>[16x]ETGDKPLGETGTTGFQICKNALKLPVLEVLPGGGWDNLRNVDMGRVMDLTYTNCKTTEDGQYIIPDEVYTIPQKESNLEMNSEVLESWMNYQSTTSLSINTELALFSRVNGKFSTEFQRMKTLQVKDQAVTTRVQVRNRIYTVKTTPTSELSLGFTKALMDICDQLEKNQTKMATYLAELLILNYGTHVITSVDAGAALVQEDHVRSSFLLDNQNSQNTVTASAGIAFLNIVNFKVETDYISQTSLTKDYLSNRTNSRVQSFGGVPFYPGITLETWQKGITNHLVAIDRAGLPLHFFIKPDKLPGLPGPLVKKLSKTVETAVRHYYTFNTHPGCTNVDSPNFNFQANMDDDSCDAKVTNFTFGGVYQECTELSGDVLCQNLEQKNLLTGDFSCPPGYSPVHLLSQTHEEGYSRLECKKKCTLKIFCKTVCEDVFRVAKAEFRAYWCVAAGQVPDNSGLLFGGVFTDKTINPMTNAQSCPAGYIPLNLFESLKVCVSLDYELGFKFSVPFGGFFSCIMGNPLVNSDTAKDVRAPSLKKCPGGFSQHLAVISDGCQVSYCVKAGIFTGGSLLPVRLPPYTKPPLMSQVATNTVIVTNSETARSWIKDPQTNQWKLGEPLELRRAMTVIHGDSNGMSGGGTKTETSQVAPA

Perforin‐2 (PFN2, MPEG1) is a key pore‐forming protein in mammalian innate immunity restricting intracellular bacteria proliferation. It forms a membrane‐bound pre‐pore complex that converts to a pore‐forming structure upon acidification; but its mechanism of conformational transition has been debated. PFN2 belongs to the membrane attack complex‐perforin (MACPF) family and shares structural homology with bacterial cholesterol‐dependent cytolysins (CDCs; Gilbert et al, 2013). Distinct from MAC and perforin‐1, PFN2 is a type I transmembrane protein that is expected to be cleaved from its transmembrane anchor during bacterial restriction, releasing from the host membrane an ectodomain consisting of the MACPF and membrane‐binding P2 domain (McCormack & Podack, 2015).

Pore‐forming assemblies were prepared from pre‐pore oligomers pre‐assembled at pH 5.5, in which condition the bulk of the oligomers are complete full rings (Ni et al, 2020), and subsequently by lowering the pH to 3.6–4.0 in the presence of 0.056% Cymal‐6 (Ni et al, 2020). The isolated converted pores exist in two major conformations, a flat ring conformation (68.5%) and a twisted conformation (15.5%; Figs 3 and EV2), both structures comprising 16 mPFN2 subunits. The twisted pore was resolved at ~ 4 Å with local resolutions ranging from 3.4 to 9.1 Å (Fig EV3). The twisted pore is slightly larger than the flat ring pore, due partly to a break in the β‐strand packing between subunits at the cracking interface, the inner diameter being ~ 90 Å (measured between two subunits at the top of MACPF domain). Compared with the flat pore, the twisted mPFN2 pore shows a non‐perfect helical conformation with an accumulated rise of the β‐strands by 63 Å. The conformations of mPFN2 subunits in the twisted pore are almost identical to those found in the flat pore (pairwise root mean square deviation (RMSD) = 0.085 to 1.204 Å), although the transmembrane β‐hairpins in the MACPF domain bend more towards the pore interior. The intersubunit hydrogen‐bonding register of the twisted pore remains unchanged (purple lines), indicating that the accumulated rise is caused by a mild twist of the β‐barrel rather than a shift in hydrogen bond register between adjacent subunits. The plasticity of the transmembrane β‐hairpins therefore determines the structural variation in pores, suggesting a relatively straightforward conversion can be made from twisted to flat forms of the pores (Movie EV3); the twisted form may therefore constitute a transition state for pore formation by complete rings of subunits, or alternatively could be an independently‐functioning pore‐forming state of the PFN2 oligomer. The twisted form also shows a mismatch in the detergent belt, which corresponds to the position of the lipid bilayer with respect to a membrane‐inserted form of this oligomer.>[2x]MRVLIVKTSSMGDVLHTLPALTDAQQAIPGIKFDWVVEEGFAQIPSWHAAVERVIPVAIRRWRKAWFSAPIKAERKAFREALQAKNYDAVIDAQGLVKSAALVTRLAHGVKHGMDWQTAREPLASLFYNRKHHIAKQQHAVERTRELFAKSLGYSKPQTQGDYAIAQHFLTNLPTDAGEYAVFLHATTRDDKHWPEEHWRELIGLLADSGIRIKLPWGAPHEEERAKRLAEGF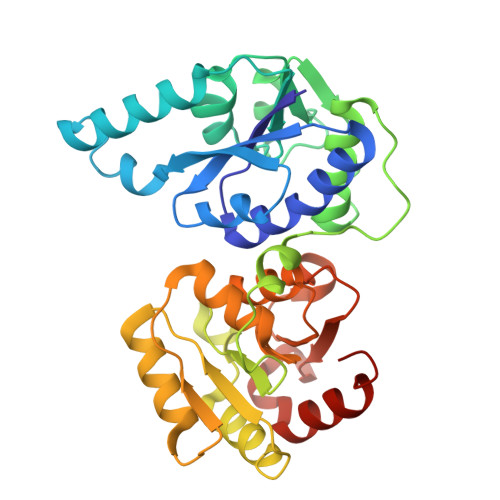AYVEVLPKMSLEGVARVLAGAKFVVSVDTGLSHLTAALDRPNITVYGPTDPGLIGGYGKNQMVCRAPGNELSQLTANAVKQFIEENAEKAAMI>MGQIVTFFQEVPHVIEEVMNIVLIALSVLAVLKGLYNFATCGLVGLVTFLLLCGRSCTTSLYKGVYELQTLELNMETLNMTMPLSCTKNNSHHYIMVGNETGLELTLTNTSIINHKFCNLSDAHKKNLYDHALMSIISTFHLSIPNFNQYEAMSCDFNGGKISVQYNLSHSYAGDAANHCGTVANGVLQTFMRMAWGGSYIALDSGRGNWDCIMTSYQYLIIQNTTWEDHCQFSRPSPIGYLGLLSQRTRDIYISRRLL[3x];>[3x]GTFTWTLSDSEGKDTPG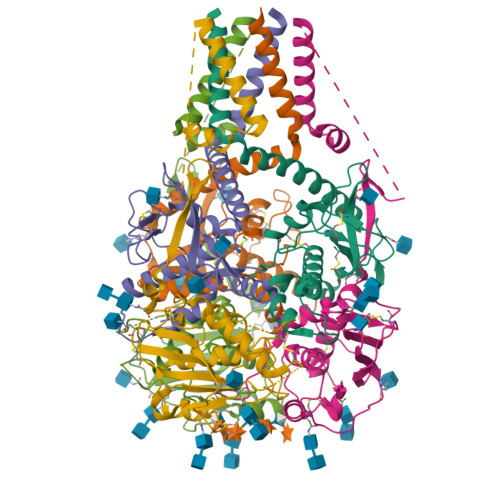GYCLTRWMLIEAELKCFGNTAVAKCNEKHDEEFCDMLRLFDFNKQAIQRLKAEAQMSIQLINKAVNALINDQLIMKNHLRDIMGIPYCNYSKYWYLNHTTTGRTSLPKCWLVSNGSYLNETHFSDDIEQQADNMITEMLQKEYMERQGKTPLGLVDLFVFSTSFYLISIFLHLVKIPTHRHIVGKSCPKPHRLNHMGICSCGLYKQPGVPVKWKRGGGSDYKDDDDK>AVKGLGKPDQVYDGSKIRVGIIHARWNRVIIDALVKGAIERMASLGVEENNIIIETVPGSYELPWGTKRFVDRQAKLGKPLDVVIPIGVLIKGSTMHFEYISDSTTHALMNLQEKVDMPVIFGLL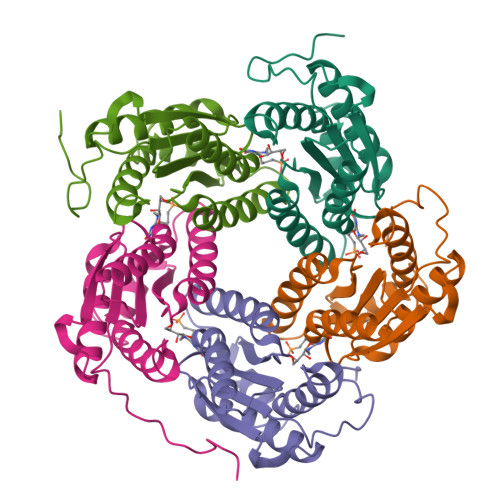TCMTEEQALARAGIDEAHSMHNHGEDWGAAAVEMAVKFGKNAF[5x]> MEATLEQRPFPYLATEANLLTQIKESAADGLFKSFQLLLGKDAREGSVRFEALLGVYTNVVEFVKFLETALAAACVNTEFKDLRRMIDGKIQFKISMPTIAHGDGRRPNKQRQYIVMKACNKHHIGAEIELAAADIE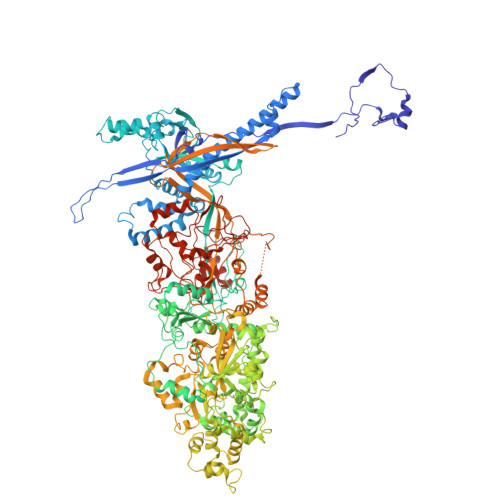LLFAEKETPLDFTEYAGAIKTITSALQFGMDALERGLVDTVLAVKLRHAPPVFILKTLGDPVYSERGLKKAVKSDMVSMFKAHLIEHSFFLDKAELMTRGKQYVLTMLSDMLAAVCEDTVFKGVSTYTTASGQQVAGVLETTDSVMRRLMNLLGQVESAMSGPAAYASYVVRGANLVTAVSYGRAMRNFEQFMARIVDHPNALPSVEGDKAALADGHDEIQRTRIAASLVKIGDKFVAIESLQRMYNETQFPCPLNRRIQYTYFFPVGLHLPVPRYSTSVSVRGVESPAIQSTETWVVNKNNVPLCFGYQNALKSICHPRMHNPTQSAQALNQAFPDPDGGHGYGLRYEQTPNMNLFRTFHQYYMGKNVAFVPDVAQKALVTTEDLLHPTSHRLLRLEVHPFFDFFVHPCPGARGSYRATHRTMVGNIPQPLAPREFQESRGAQFDAVTNMTHVIDQLTIDVIQETAFDPAYPLFCYVIEAMIHGQEEKFVMNMPLIALVIQTYWVNSGKLAFVNSYHMVRFICTHMGNGSIPKEAHGHYRKILGELIALEQALLKLAGHETVGRTPITHLVSALLDPHLLPPFAYHDVFTDLMQKSSRQPIIKIGDQNYDNPQNRATFINLRGRMEDLVNNLVNIYQTRVNEDHDERHVLDVAPLDENDYNPVLEKLFYYVLMPVCSNGHMCGMGVDYQNVALTLTYNGPVFADVVNAQDDILLHLENGTLKDILQAGDIRPTVDMIRVLCTSFLTCPFVTQAARVITKRDPAQSFATHEYGKDVAQTVLVNGFGAFAVADRSREAAETMFYPVPFNKLYADPLVAATLHPLLANYVTRLPNQRNAVVFNVPSNLMAEYEEWHKSPVAAYAASCQATPGAISAMVSMHQKLSAPSFICQAKHRMHPGFAMTVVRTDEVLAEHILYCSRASTSMFVGLPSVVRREVRSDAVTFEITHEIASLHTALGYSSVIAPAHVAAITTDMGVHCQDLFMIFPGDAYQDRQLHDYIKMKAGVQTGPPGNRMDHVGYAAGVPRCENLPGLSHGQLATCEIIPTPVTSDVAYFQTPSNPRGRAACVVSCDAYSNESAERLLYDHSIPDPAYECRSTNNPWASQRGSLGDVLYNITFRQTALPGMYSPCRQFFHKEDIMRYNRGLYTLVNEYSARLAGAPATSTTDLQYVVVNGTDVFLDQPCHMLQEAYPTLAASHRVMLDEYMSNKQTHAPVHMGQYLIEEVAPMKRLLKLGNKVVY> MATTNYFKVKLLDEKLIPFLGLGERGPRENVILSSNDLASLKQAGWTVTDVQPLPETGKIKYDRRTVYFKSEGETGKFINVPFYINPVDARDVLGLLKFDLIKLSDKSVVKTYTAKDIKSEILSLPTSDLEVNEEYELKLYFPKDASENYDIAISEGHKNLFERVKDSVFIKVKEYGKFTGRLVQLQQDINVLKESALPLDKILGYKDFDTKEVTPVAKENLLQLLSVNVSDESYARYQADKNR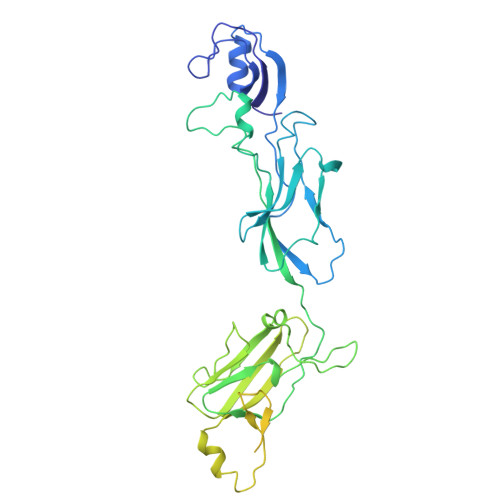LLFFSKTGEILVKVIERSIQDNIVNFNIRILDEETIQNEIDKKIEYSVYDPKDGKFESINQTKSITVTPETVNIEAEQTQKLEVTTEPEGRKVSFELKDGSEFASVDNNGNITGISEGTANVTVKSDDVSKNVEVNVSRLKTKSLTVTPEEVNIDAESTQQLDVKIQPSTNSVSYSITEGSEYASVNNSGLVTAKAAGTAKVKVTSDSVSKDVSVTISTSQVEETPEETTTE> GSGSGDVMRRRIATPEEVRLPLQHGWRREVRIKKGSHRWQGETWYYGPCGKRMKQFPEVIKYLSRNVVHSVRREHFSFSPRMPVGDFFEERDTPEGLQWVQLSAEEI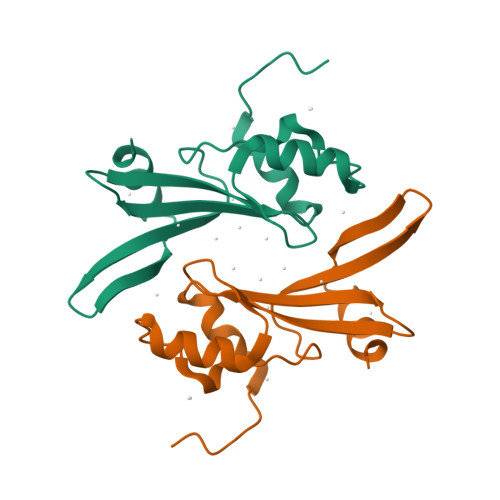PSRIQAITGKRG>MRGSHHHHHHGSKKGDLVAWNKENDRRTLWTTPDPSPNCKVSEEKDSKLTLVLTKCGSQILASVSLLVVKGKFANINNKTNPGEDYKKFSVKLLFDANGKLLTGSSLDGNYWNYKNKDSVIGSPYENAVPFMPNS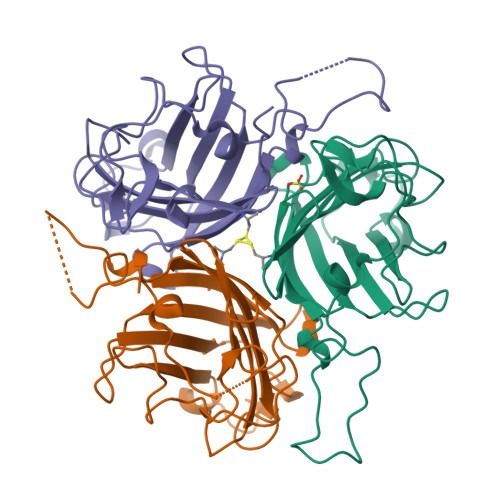TAYPKIINNGTANPEDKKSAAKKTIVTNVYLGGDAAKPVATTISFNKETESNCVYSITFDFAWNKTYKNVPFDSSSLTFSYIAQDAEDKNE[6x]> STRDYEIQRERIELGRCIGEGQFGDVHQGIYMSPENPAMAVAIKTCKNCTSDSVREKFLQEALTMRQFDHPHIVKLIGVITENPVWIIMELCTLGELRSFLQVRKYSLDLASLILYAYQLSTALAYLESKRFVHRDIAARNVLVSSNDCVKLGDFGLSRYMEDSTYYKASKGKLPIKWMAPESINFRRFTSASDVWMFGVCMWEILMHGVKPFQGVKNNDVIGRIENGERLPMPPNCPPTLYSLMTK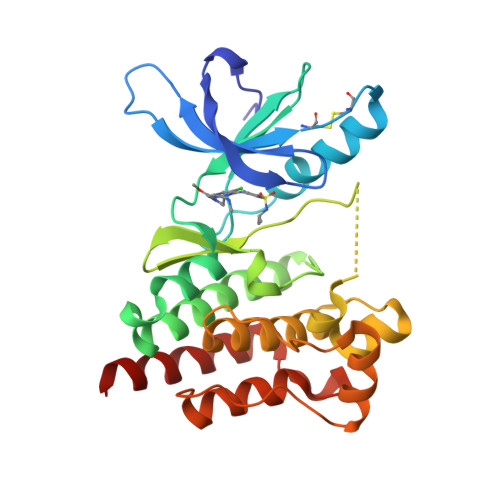CWAYDPSRRPRFTELKAQLSTILEEEKLQ3-[(1S,2S)-2-(7-hydroxy-1H-benzimidazol-2-yl)cyclopentyl]benzoic acid | C19 H18 N2 O3 | 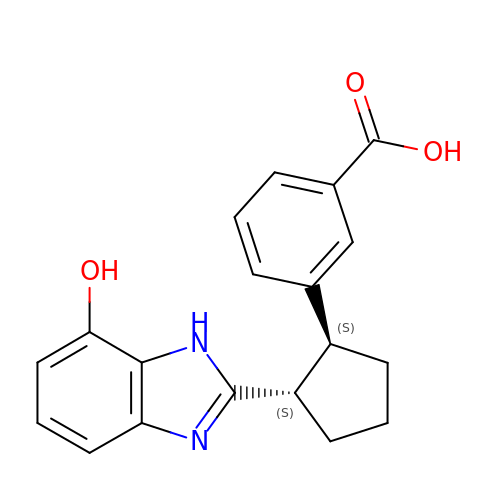HDENXLNFCHSDIF-KGLIPLIRSA-N> STLTE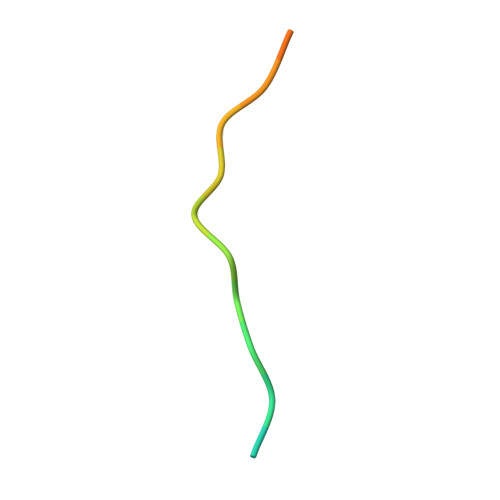EFELLISNSEDDWE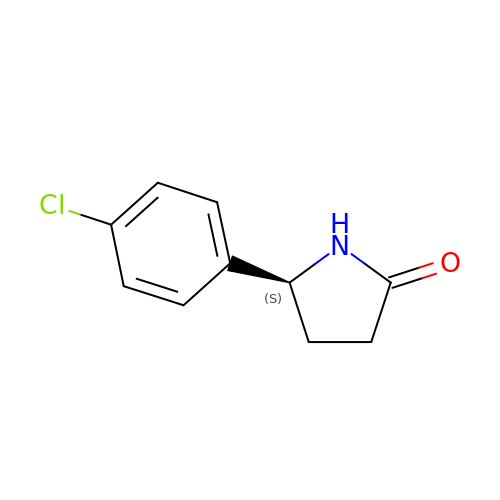(5~{S})-5-(4-chlorophenyl)pyrrolidin-2-one | C10 H10 Cl N O | BSYBLMDNOUEPRW-VIFPVBQESA-N> SSLDDKPQFPGASAEFIDKLEFIQPNVISGIPIYRVMDRQGQIINPSEDPHLPKEKVLKLYKSMTLLNT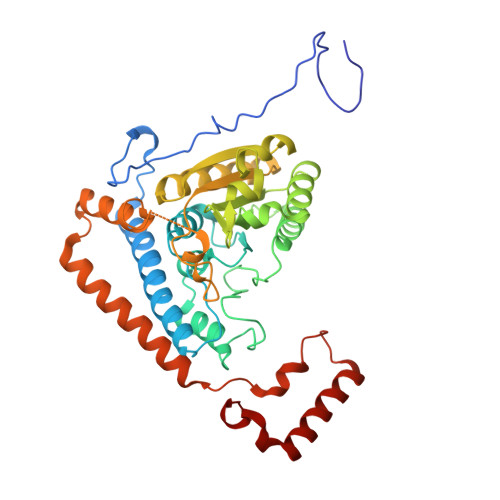MDRILYESQRQGRISFYMTNYGEEGTHVGSAAALDNTDLVFGQYREAGVLMYRDYPLELFMAQCYGNISDLGKGRQMPVHYGCKERHFVTISSPLATQIPQAVGAAYAAKRANANRVVICYFGEGAASEGDAHAGFNFAATLECPIIFFCRNNGYAISTPTSEQYRGDGIAARGPGYGIMSIRVDGNDVFAVYNATKEARRRAVAENQPFLIEAMTYRIGHHSTSDDSSAYRSVDEVNYWDKQDHPISRLRHYLLSQGWWDEEQEKAWRKQSRRKVMEAFEQAERKPKPNPNLLFSDVYQEMPAQLRKQQESLARHLQTYGEHYPLDHFDK> MSQQSSSPTKEDNNSSSPVVPNPDSVPPQLSSPALFYSSSSSQGDIYGRNNSQNLSQGEGNIRAAIGSSPLNFPSSSQRQNSDVFQSQGRQGRIRSSASASGRSRYHSDLRSDRALPTSSSSLGRNGQNRVHMRRNDIHTSDLSSPRRIVDFDTRSGVNTLDTSSSSAPPSEASEPLRIIWGTNVSIQECTTNFRNFLMSFKYKFRKILDEREEFINNTTDEELYYIKQLNEMRELGTSNLNLDARNLLAYKQTEDLYHQLLNYPQEVISIMDQTIKDCMVSLIVDNNLDYDLDEIETKFYKVRPYNVGSCKGMRELNPNDIDKLINLKGLVLRSTPVIPDMKVAFFKCNVCDHTMAVEIDRGVIQEPARCERIDCNEPNSMSLIHNRCSFADKQVIKLQETPDFVPDGQTPHSISLCVYDELVDSCRAGDRIEVTGTFRSIPIRANSRQRVLKSLYKTYVDVVHVKKVSDKRLDVDTSTIEQELMQNKVDHNEVEEVRQITDQDLAKIREVAAREDLYSLLARSIAPSIYELEDVKKGILLQLFGGTNK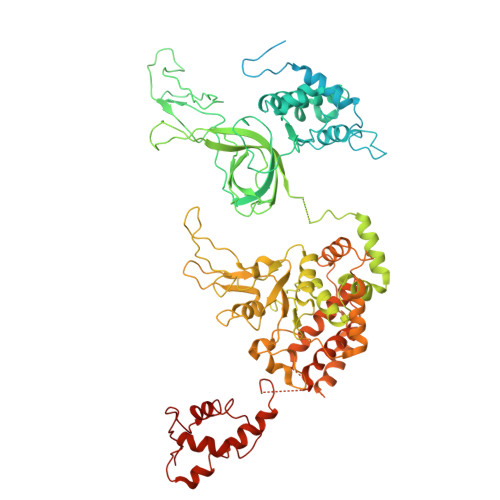TFTKGGRYRGDINILLCGDPSTSKSQILQYVHKITPRGVYTSGKGSSAVGLTAYITRDVDTKQLVLESGALVLSDGGVCCIDEFDKMSDSTRSVLHEVMEQQTISIAKAGIITTLNARSSILASANPIGSRYNPNLPVTENIDLPPPLLSRFDLVYLVLDKVDEKNDRELAKHLTNLYLEDKPEHISQDDVLPVEFLTMYISYAKEHIHPIITEAAKTELVRAYVGMRKMGDDSRSDEKRITATTRQLESMIRLAEAHAKMKLKNVVELEDVQEAVRLIRSAIKDYATDPKTGKIDMNLVQTGKSVIQRKLQEDLSREIMNVLKDQASDSMSFNELIKQINEHSQDRVESSDIQEALSRLQQEDKVIVLGEGVRRSVRLNNRV>MARQLRAEQTRATIIGAAADLFDRRGYESTTLSEIVAHAGVTKGALYFHFAAKEDLAHAILEIQSRTSRRLAKDLDGRGYSSLEALMRLTFGMARLCVQGPVLRAGLRLATAGVPVRPPLPHPFTEW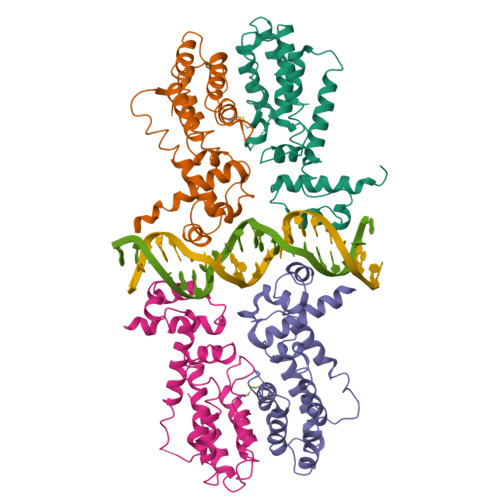REIATSRLLDAVRQSDVHQDIDVDSVAHTLVCSVVGTRVVGGTLEPAGREPRRLAEMWYILIRGMVPVTRRARYVTLAARLEQETGTA[4x]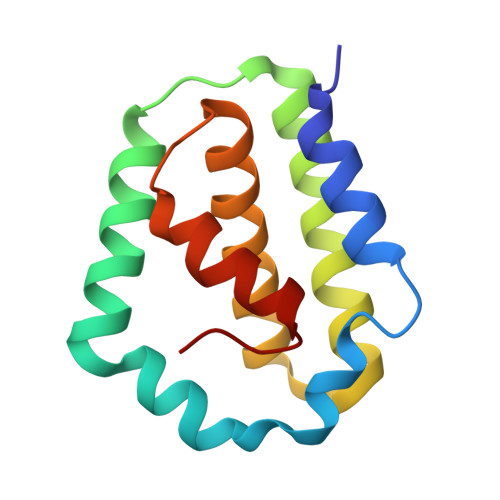> MINNKLIEIDNCLSAPSFFDFLKSLNVDSALDSRDEPEFDDCWMSEFNSLDKESFQDDDIEFIDSLREKAFKYSFRVINNAEISSRISDDIEIISKSFVLEKENSWSITHLWSSYKNGKFPE>GSHMSQSFGRVLTIVHSDCALLERDGNISLLSLPVAERWLRQAQLTPGEAPVCAQPLLIPLRLKVSAEEKSALEKAQSALAELGIDFQSDAQHVTIRAVPLPLRQQNLQILIPELIGYLAKQSVFEPGNIAQWIARNLMSEHAQWSMAQAITLLADVERLCPQLVKTPPGGLLQSVDLH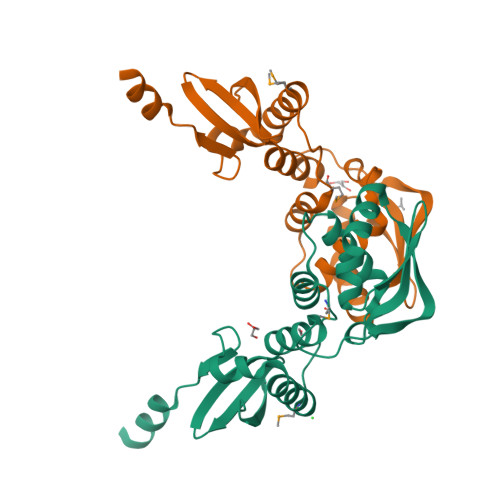PAIKALKDE[2x]>MSLLIRGATVVTHEESYRADVLCANGLIQAIGENLETPSGCDVLDGGGQYLMPGGIDPHTHMQLPFMGTVASEDFFSGTAAGLAGGTTSIIDFVIPNPRQSLLEAFHTWRGWAQKSAADYGFHVAITWWSDEVAREMGELVAQHGVNSFKHFMAYKNAIMAADDTLVASFERCLELGAVPTVHAENGELVFHLQQKLLAQGLTGPEAHPLSRPPQVEGEAASRAIRIAETLGTPLYLVHISSREALDEIAYARAKGQPVYGEVLAGHLLLDDSVYRHPDWATAAGYVMSPPFRPVEHQEALWRGLQSGNLHTTATDHCCFCAEQKAMGRDDFSKIPNG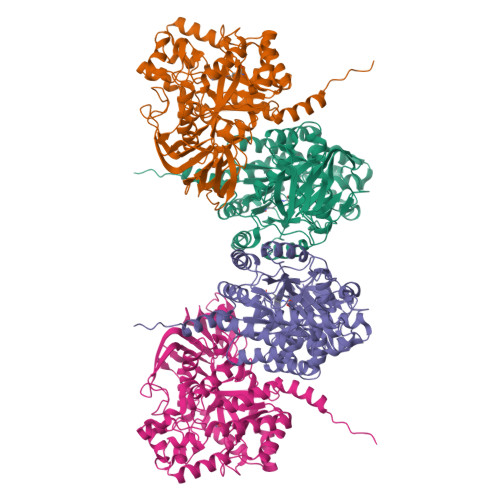TAGIEDRMALLWDAGVNSGRLSMHEFVALTSTNTAKIFNLFPRKGAIRVGADADLVLWDPQGSRTLSAATHHQRVDFNIFEGRTVRGIPSHTISQGKLLWAAGDLRAEPGAGRYVERPAYPSVYEVLGRRAERQRPVAVER[4x]> APIDDQLAELERRDNVLIGLYAANLQSGRRITHRPDEMFAMCSTFKGYVAARVLQMAEHGEISLDNRVFVDADALVPNSPVTEARAGAEMTLAELCQAALQRSDNTAANLLLKTIGGPAAVTAFARSVGDERTRLDRWEVELNSAIPGDPRDTSTPAALAVGYRAILAGDALSPPQRGLLEDWMRANQTSSMRAGLPEGWTTADKTGSGDYGSTNDAGIAFGPDGQ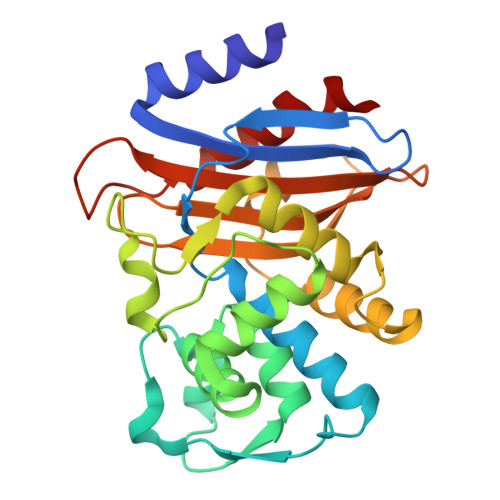RLLLVMMTRSQAHDPKAENLRPLIGELTALVLPSLL>GSHMIQAYLGLGSNIGDRESQLNDAIKILNEYDGISVSNISPIYETAPV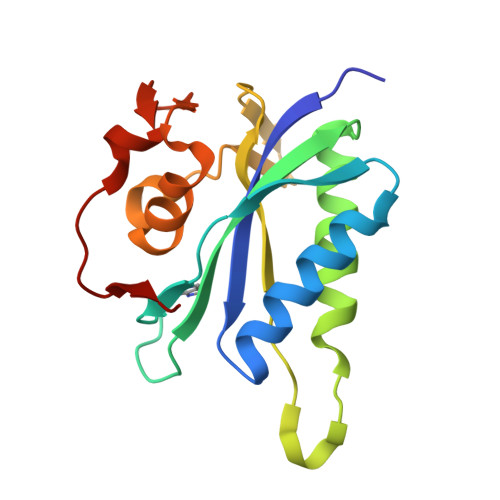GYTEQPNFLNLCVEIQTTLTVLQLLECCLKTEECLHRIRKERWGPRTLDVDILLYGEEMIDLPKLSVPHPRMNERAFVLIPLNDIAANVVEPRSKLKVKDLVFVDDSVKRYK[2x]> RSPWCVICDPSVVLALKSLEKDYLPGHLDAKHHKAMMERVENAVKDFQELSLNEDAYMGVVDEATLQKGSWSLLKDLKRITDSDVKGDLFVKELFWMLHLQKETFATYVARFQKEAYCPNKCGVMLQTLIWCKNCKKEVHACRKSYDCGERNVEVPQMEDMILDCELNWHQASEGLTDYSFYRVWGNNTETLVSKGKEATLTKPMVGPEDAGSYRCELGSVNSSPATIINFHVTVLPKEFLEVLFQ;> RSPWGDELLNICMNAKHHKRVPSPEDKLYE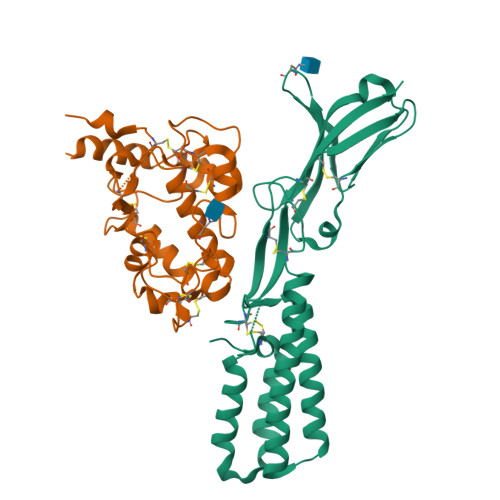ECIPWKDNACCTLTTSWEAHLDVSPLYNFSLFHCGLLMPGCRKHFIQAICFYECSPNLGPWIQPVGSLGWEVAPSGQGERVVNVPLCQEDCEEWWEDCRMSYTCKSNWRGGWDWSQGKNRCPKGAQCLPFSHYFPTPADLCEKTWSNSFKASPERRNSGRCLQKWFEPAQGNPNVAVARLFASEFLEVLFQ> MKILILGIFLFLCSTPAWAKEKHYYIGIIETTWDYASDHGEKKLISVDTEHSNIYLQNGPDRIGRLYKKALYLQYTDETFRTTIEKPVWLGFLGPIIKAETGDKVYVHLKNLASRPYTFHSHGITYYKEHEGAIYPDNTTDFQRADDKVYPGEQYTYMLLATEEQSPGEGDGNCVTRIYHSHIDAPKDIASGLIGPLIICKKDSLDKEKEKHIDREFVVMFSVVDENFSWYLEDNIKTYCSEPEKVDKDNEDFQESNRMYSVNGYTFGSLPGLSMCAEDRVKWYLFGMGNEVDVHAAFFHGQALTNKNYRIDTINLFPATLFDAYMVAQNPGEWMLSCQNLNHLKAGLQAFFQVQECNKSSSKDNIRGKHVRHYYIAAEEIIWNYAPSGIDIFTKENLTAPGSDSAVFFEQGTTRIGGSYKKLVYREYTDASFTNRKERGPEEEHLGILGPVIWAEVGDTIRVTFHNKGAYPLSIEPIGVRFNKNNEGTYYSPNYNPQSRSVPPSASHVAPTETFTYEWTVPKEVGPTNADPVCLAKMYYSAVDPTKDIFTGLIGPMKICKKGSLHANGRQKDVDKEFYLFPTVFDENESLLLEDNIRMFTTAPDQVDKEDEDFQESNKMHSMNGFMYGNQPGLTMCKGDSVVWYLFSAGNEADVHGIYFSGNTYLWRGERRDTANLFPQTSLTLHMWPDTEGTFNVECLTTDHYTGGMKQKYTVNQCRRQSEDSTFYLGERTYYIAAVEVEWDYSPQREWEKELHHLQEQNVSNAFLDKGEFYIGSKYKKVVYRQYTDSTFRVPVERKAEEEHLGILGPQLHADVGDKVKIIFKNMATRPYSIHAHGVQTESSTVTPTLPGETLTYVWKIPERSGAGTEDSACIPWAYYSTVDQVKDLYSGLIGPLIVCRRPYLKVFNPRRKLEFALLFLVFDENESWYLDDNIKTYSDHPEKVNKDDEEFIESNKMHAINGRMFGNLQGLTMHVGDEVNWYLMGMGNEIDLHTVHFHGHSFQYKHRGVYSSDVFDIFPGTYQTLEMFPRTPGIWLLHCHVTDHIHAGMETTYTVLQNEDTKSG

Human ceruloplasmin (Cp) is a multi-functional copper-containing protein. Indeed, Cp oxidizes highly toxic ferrous ions to the ferric state for further incorporation into apo-transferrins, catalyzes Cu(I) oxidation and promotes the oxidation of biogenic amines (norepinephrine, serotonin) and synthetic amines (p-phenylenediamine (p-PD), o-dianisidine(o-DA)). The Cp molecule (∼132 kDa) consists of a single polypeptide chain with 1046 amino acid residues. Mpo (EC 1.11.1.7) is one of the major proteins of the antimicrobial system of mammalian neutrophils.

A re-refined structure of Cp at 2.6 Å was employed for construction of models, elucidation of additional details of the structural organization of Cp, and for comparative analysis. However, it was not possible to unambiguously trace the majority of interdomain linking regions most likely because of their inherent flexibility (these linkers have thus not been included in the present model). Domains 2, 4, and 6 contained one type I copper each. Three copper ions (two type III and one type II) form a trinuclear cluster with ligands provided by domains 1 and 6. The structure of Cp contains five disulfide bridges stabilizing the external loops between the β-strands. The S-S bridge between Cys881 and Cys885 is not the only factor that stabilizes the interdomain loop 885–893, but the end of this loop is additionally stabilized via H-bonds of Arg893 with Asp959 based on the our Cp structure. The H-bond network links two different β-sheets, but also restricts the loop end movements in case of proteolysis that results in cleavage of the bond next to Arg893. Another binding site was located in domain 4 of Cp near the side chain of Trp669. Amino acids in domain 4 of Cp localized in close proximity to the p-PD-binding site are involved in the contact. This binding site in the Cp molecule includes amino acid residues His667 and Trp669 and also Ser622, as demonstrated in the present work.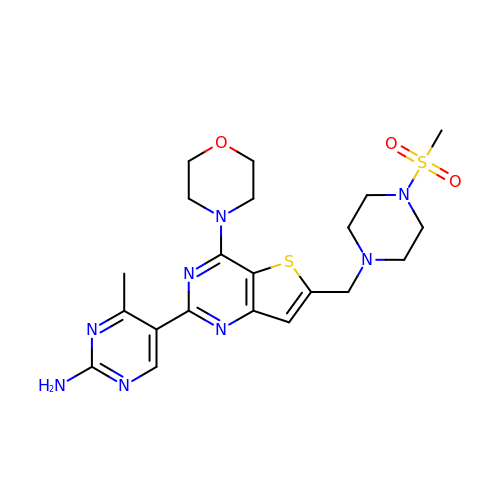4-methyl-5-(6-{[4-(methylsulfonyl)piperazin-1-yl]methyl}-4-morpholin-4-ylthieno[3,2-d]pyrimidin-2-yl)pyrimidin-2-amine | C21 H28 N8 O3 S2 | XAZDYPNMXGDMSA-UHFFFAOYSA-N1-methylcyclobutyl [(2R,6S,12Z,13aS,14aR,16aS)-2-[(7-methoxy-3-methylquinoxalin-2-yl)oxy]-14a-{[(1-methylcyclopropyl)sulfonyl]carbamoyl}-5,16-dioxo-1,2,3,5,6,7,8,9,10,11,13a,14,14a,15,16,16a-hexadecahydrocyclopropa[e]pyrrolo[1,2-a][1,4]diazacyclopentadecin-6-yl]carbamate 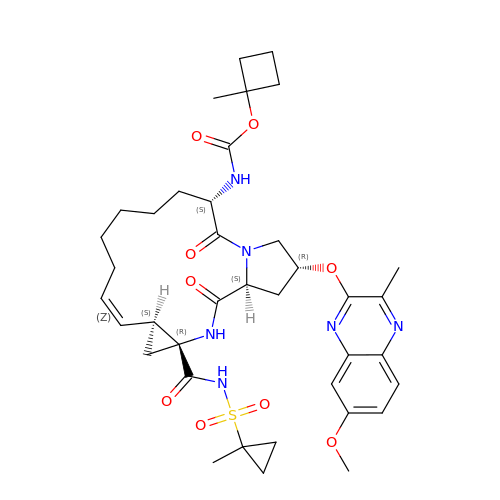| C38 H50 N6 O9 S | PDBMENIRROXLPP-AJUMDJHNSA-N>[2x]MSTDIDCIVIGAGVVGLAIARALAAGGHEVLVAEAAEGIGTGTSSRNSEVIHAGIYYPADSLKARLCVRGKHLLYEYCAARGVPHQRLGKLIVATSDAEASQLDSIARRAGANGVDDLQHIDGAAARRLEPALHCTAALVSPSTGIVDSHALMLAYQGDAESDGAQLVFHTPLIAGRVRPEGGFELDF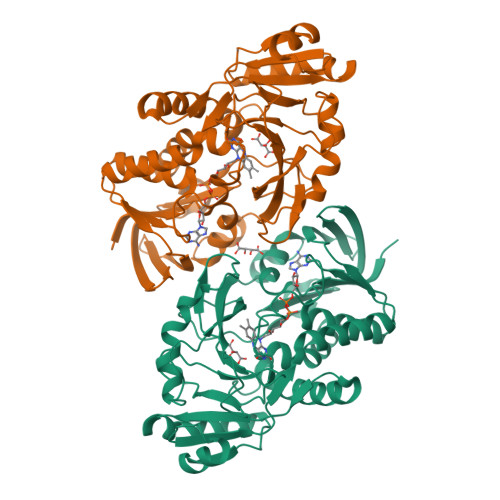GGAEPMTLSCRVLINAAGLHAPGLARRIEGIPRDSIPPEYLCKGSYFTLAGRAPFSRLIYPVPQHAGLGVHLTLDLGGQAKFGPDTEWIATEDYTLDPRRADVFYAAVRSYWPALPDGALAPGYTGIRPKISGPHEPAADFAIAGPASHGVAGLVNLYGIESPGLTASLAIAEETLARLAA>MVLNSNELEHIHSTNHSVNDISIRWGVIGAGQKGNKEADLFAGYKFSNGTTCYPTLAVNFAESDMMHLQNIIKEDRIHFDGLKGAARTPSVVTDLFDPETNPNANGYLDKLAQELGRKFTNEEGEVIVDQFLICLGAGGGVGTGWGSLVLQLIREQFFPCPVSMLISLPSGDPDEINNALVLLSEIDEFMREQDRLFGNSDIKPLANVIVNDNTQMQRIIESQKGTKDLKNRYVNWKEVANDNVVSTLHEINIIPENYGSDNVTYDPSDLIKLLSIPGRFLTIGKARIAKFDLHSLENSIKRSLDEGFFSAEHQFETATMYGGFVLRPSNADFFKDVNTENRIRNTLGEYKRLDEIAGKFGDPI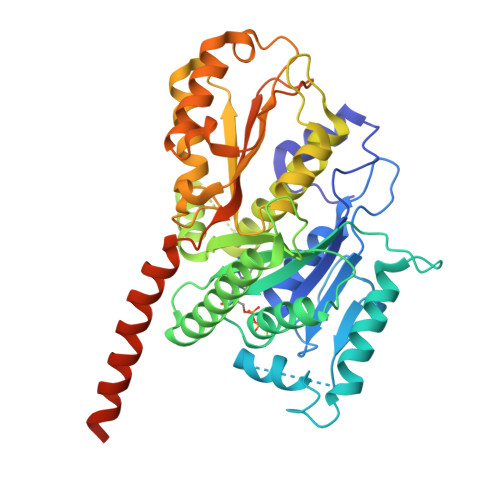WDNEYAVCYTIFAGMTMPKRYISLAREGKELAEKQEQLRAEAQRKQDEEKVDISFATHHHHHH[12x]>MFQMSETERTLVIIKPDAVVRGLIGEIISRFEKKGLKIVGMKMIWIDRELAEKHYEEHREKPFFKALIDYITKTPVVVMVLEGRYAVEVVRKMAGATDPKDAAPGTIRGDFGLEVSDAICNVIHASDSKESAEREISLFFKPEELFEYPRAADW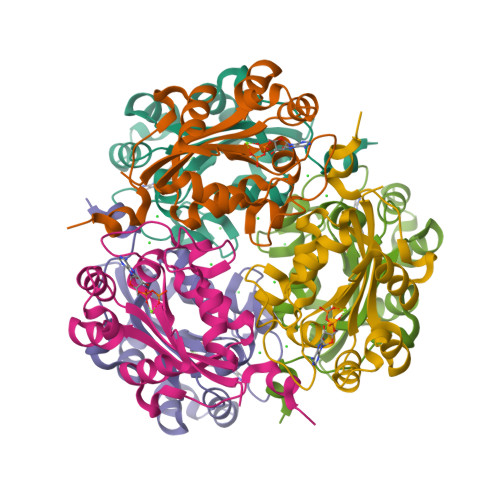FYKKGI[2x]> SMETLD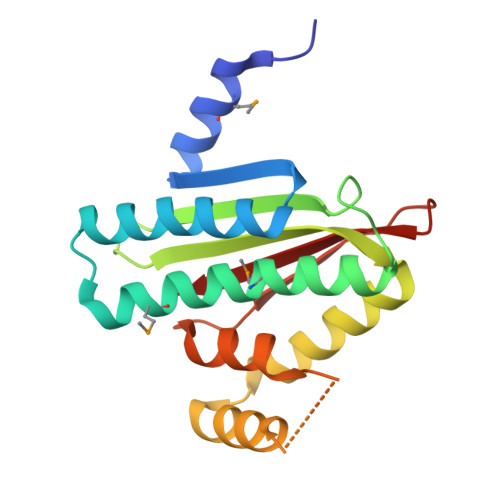LLAMRESYTRQRILLCFNGPISRSLIEEIGHALRNYLHAEQAKPSEAMDVFAVYIEMTQNIRHYANLKGYGEHEAAATVAIARNEDGHYVVSAGNLVERDDGQSLVRSIQAIANLDKAALKAAYKEQLRRPRDSGCASGAGLGLLDIARKSSEPLAASLKEQPDGRAFFSLRAVI>FGDLSGIISRDQFYKMLKHMNDNDCHAVGFFTYDAFITAAKSFPSFGNTGDLAMRKKEIAAFFGQTSHETTGGWSGAPDGANTWGYCYKEAIDKSDPHCDSNNLEWPCAPGKFYYGRGPMMLSWNYNYGPCGRDLGLELL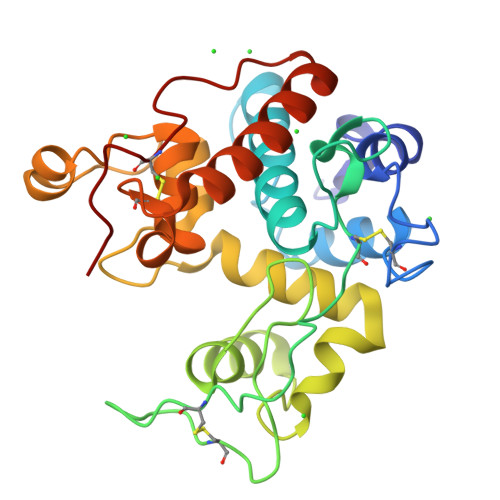KNPDVASSDPVIAFKTAIWFWMTPQAPKPSCHDVITDQWEPSAADISAGRLPGYGVITNIINGGLECAGRDVAKVQDRISFYTRYCGMFGVDPGSNIDCDNQRPFN[2x]> ETGKPSFVTFRGEPAEGFNHLVVDERTGHIYLGAVNRIYKLSSDLKVLVTHQTGPDEDNPKCYPPRIVQTCNEPLASTNNVNKMLLIDYKENRLIACGSLYQGICKLLRLEDLFKLGEPFHKKEHYLSGVNESGSVFGVIVSYSNFDDKLFIATAVDGKPEYFPTISSRKLTKNSEADGMFAYVFHDEFVASMIKIPSDTFTVIPDFDIYYVYGFSSGNFVYFLTLQPEMVSPPGSTTKEQVYTSKLVRLCKEDTAFNSYVEVPIGCERNGVEYRLLQAAYLSKAGAVLGRTLGVRPDDDLLFTVFSKGQKRKMKSLDESALCIFILKQINDRIKDRLQSCYRGEGTLDLAWLKVKDIPCSSALLTIDDNFCGLDMNAPLGVSEMVRGIPVFTEDRDRMTSVIAYVYKNHSLAFVGTKSGKLKKIRVDGPKGNALQYETVQVVDSGPVLRDMAFSKDHEQLYIMSERQLTRVPVESCGQYRSCGECLGSGDPHCGWCVLHNTCTRKERCERSREPRRFASEMKQCVRLTVHPNNISVSQYNVLLVLETYNVPELSAGVNCTFEDLSEMDGLVIGNQIQCYSPAAKEVPRIITENGDHHVVQLQLKSKETGMTFASTSFVFYNCSVHNSCLSCVESPYRCHWCKYRHVCTHDPNTCSFQEGRVKLPEDCPQLLRVDKILVPVEVIKPITLKAKNLPQPQSGQRGYECILNIQGIEQRVPALRFNSSSVQCQNTSYSYEGMEINNLPVELTVVWNGHFNIDNPAQNKVYLYKCGAMRESCGLCLKADPDFECGWCQSPGQCTLRQHCPAHESRWLELSGANSKCTNPRITEIIPVTGPREGGTKVTIRGENLGLEFRDIASHVKVAGVECSPLVDGYIPAEQIVCEMGEAKPSQHAGFVEICVAVCRPEFMARSSQLYYFMTLTLADLKPNRGPMSGGTQVTITGTNLNAGSNVVVMFGSQPCLFHRRSPSYIICNTTSSEEVLDMKVTVQVDRARIRQDLVFQYVEDPTIVRIEPEWSIVSGNTPIAVWGTHLDLIQNPQIRAKHGGKEHINICEVLNATEMTCQAPALALGPDHQSDLTERPEEFGFILDNVQSLLILNKTNFTYYPNPVFEAFSPSGILELKPGTPIILKGKNLIPPVAGGNVKLNYTVLVGEKPCTVTVSDVQLLCESPNLIGRHKVMARVGGMEYSPGMVYIAPGRTKHHHHHH

Class A plexins (PlxnAs) act as semaphorin receptors and control diverse aspects of nervous system development and plasticity, ranging from axon guidance and neuron migration to synaptic organization. Plexins are large type 1 transmembrane proteins comprising typically ten domains in their extracellular segment, a single membrane spanning region that is predicted to be helical and a conserved, cytoplasmic region that contains a GTPase-activating protein (GAP) domain with a Rho GTPase-binding domain insert. All our PlxnA ectodomain structures show autoinhibitory, intermolecular “head-to-stalk” (domain 1 to domain 4-5) interactions, which are confirmed by biophysical assays, live cell fluorescence microscopy, and cell-based and neuronal growth cone collapse assays. This work reveals a 2-fold role of the PlxnA ectodomains: imposing a pre-signaling autoinhibitory separation for the cytoplasmic domains via intermolecular head-to-stalk interactions and supporting dimerization-based PlxnA activation upon ligand binding.

We determined crystal structures of the full extracellular segments of mouse PlxnA1, PlxnA2, and PlxnA4 from eight crystal forms providing a total of 13 independent structures that range in maximum resolution from 4 to 10 Å. In five out of 13 full extracellular structures all ten domains are resolved whereas in the other eight structures some of the C-terminal domains were not modeled due to fragmentary or absent electron density. Some flexibility in the stalk is evident on comparison of the 13 different structures and contributes to the ring diameter ranging from 84 Å to 99 Å. The membrane proximal domain IPT6 (domain 10) is positioned perpendicular to the ring formed by domains 1 to 9, and the IPT6 C terminus points away from the plane of the ring. This out-of-the-ring orientation of IPT6 is observed in all five PlxnA ectodomain structures for which the electron density is sufficiently well ordered to allow IPT6 to be resolved. All our PlxnA full ectodomain crystal structures have an intermolecular plexin–plexin interface in common. This interface is formed by blades 1–3 of the sema domain of one plexin molecule and the outer side of domains 4-5 (PSI2-IPT2) from the ring of a second plexin. Superposition of the crystal structure for a full-length PlxnA extracellular segment onto our previously reported Sema6Aecto–PlxnA21-4 complex (Janssen et al., 2010) brings the two IPT6 domains into close proximity. The distances between the two PlxnA ectodomain C-termini in these modeled complexes range from 10 Å to 59 Å for the five PlxnA crystal structures that have all ten domains resolved.>MASASSSQRGRSGSGNFGGGRGGGFGGNDNFGRGGNFSGRGGFGGSRGGGGYGGSGDGYNGFGNDGSNFGGGGSYNDFGNYNNQSSNFGPMKGGNFGGRSSGPYGGGGQYFAKPRNQGGYGGSSSSSSYGSGRRF[6x]

Heterogeneous nuclear ribonucleoprotein A1 (hnRNPA1) is a multifunctional protein playing key roles in the regulation of gene expression and RNA metabolism. HnRNPA1 contains two globular RNA recognition motifs (RRM1 and RRM2) for the specific binding with mRNA precursor, followed by an unstructured low complexity (LC) C-terminal domain. HnRNPA1 LC consists of a cluster of RGG repeats with interspersed aromatic residues and a nuclear localization sequence (termed PY-NLS). The LC domain also exerts a prion-like function to mediate the amyloid aggregation of hnRNPA1, which is causative to neurodegenerative diseases including amyotrophic lateral sclerosis (ALS) and multisystem proteinopathy (MSP), and enhanced by inheritable mutations.

In this work, we determine the atomic structure of amyloid fibril formed by hnRNPA1 LC domain by cryo-electron microscopy (cryoEM). Recombinant hnRNPA1 LC (residues 186–320) was incubated at 16 °C for 2 days to form amyloid fibrils. We then performed helical reconstruction by Relion21 and obtained the three-dimensioanl (3D) density map of the hnRNPA1 LC fibril to an overall resolution of 2.8 Å. The density map showed two protofilaments intertwining along an approximate twofold screw axis to form a left-handed helix with a width of ~7 nm and a half pitch of ~45 nm. The helical twist and rise between neighboring hnRNPA1 LC subunits are 179.05° and 2.37 Å, respectively. Based on the high-resolution cryoEM density map, we were able to unambiguously build an atomic structure model for hnRNPA1 LC fibril. Despite that the fibrils were formed by hnRNPA1 residues 186–320, only residues 251–295 were involved in the fibril core. The structure reveals that the fibril core is mainly formed and stabilized by PY-NLS. The serpentine fold of hnRNPA1 fibril core remarkably contains a single but long β-strand composed of residues 260–273. β-Strands of the same protofilament form a parallel β-sheet with a kink at 263FG264. In the steric zipper, the opposing polar side chains of N265, N267, Q269, and S271 are tightly interdigitated to each other via van der Waals forces to form a shape complimentary dry interface, which is reminiscent of the first atomic structure of steric zipper formed by segment GNNQQNY of yeast prion Sup35. Thus, the binding of PY-NLS with Kapβ2 can directly prevent it from driving the amyloid fibril formation of hnRNPA1, which provides structural understanding for the chaperone activity of Kapβ2 in the inhibition and disaggregation of hnRNPA1 fibril formation.> MENYFQAEAYNLDKVLDE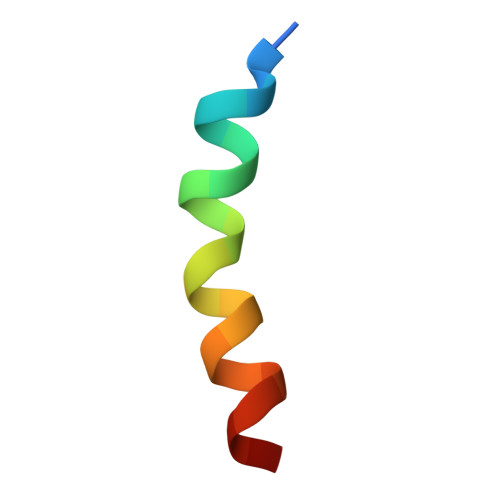FEQN> DEYSYYKLKGASTQLEYTKYMASTLQEIAQRFPDLQNTGILQDLENYNKAWNDFASNPNENATKIALVKASQTLTESVNNTFATLDKIQKKVNDDIKNTVDEINRIGEEIATINKQIYGQEALPTEHANELRDRRDELELTLSKLVSAVASKNEINQDNRLDTTITDPGHQYNLSIEGFSIVDGINFHPLKLDYDDKNKSYSIYYETPDEKVRDLTAKISGGQLGAQLDLRGRNYSKSEGKYEDGIIQGYMDSLDTFAKTMINETNNLYASSAKSSVTSDYLSGLKGDIPLVNYDRTIQPGSFDIVIYDDKGDKKLTKTITIDVNTTMNDIMRQINANTDDNDNKNSNDDVDDHINASFSYDAKTGDGLFQINAKSGFKVAIEDKGTNFAGAFSIGGFFSGTDASDMKVKDSILNDPSTVRASSNGVDSGNDMANKIIQLQYKKVNFYNEDGTIDNLTMEEYY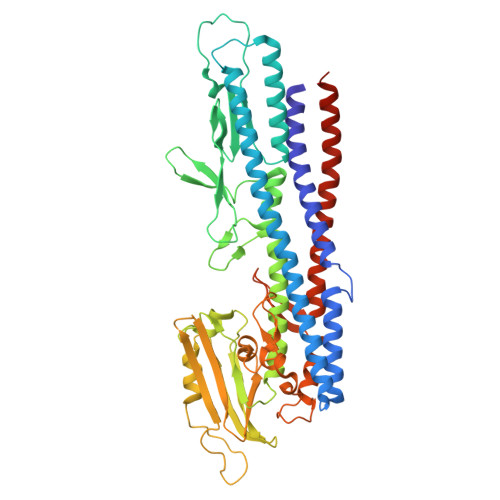RKLTGKIASDGENNNVVNSSNETLYNSVYSEYQSKSGVNTNEELAALI> MEFDDDLVDAEGNLVEAGGTYYLLPHIWAHGGGIETAKTGNEPCPLTVVRSPNEVSKGEPIRISSQFLSLFI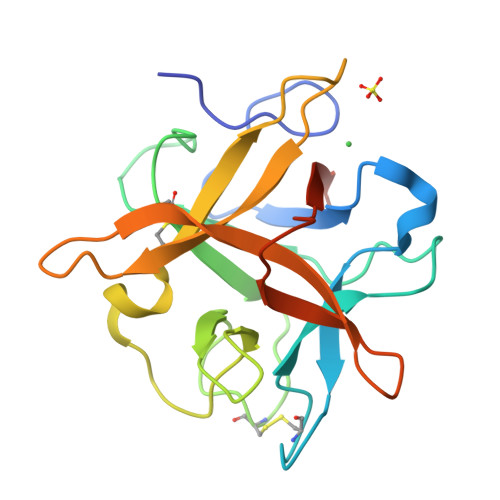PRGSLVALGFANPPSCAASPWWTVVDSPQGPAVKLSQQKLPEKDILVFKFEKVSHSNIHVYKLLYCQHDEEDVKCDQYIGIHRDRNGNRRLVVTEENPLELVLLKAKSETASSH> DPDVDECQLMPNACQNGGTCHNSHGGYNCVCVNGWTGEDCSENIDDCASAACFQGATCHDRVASFYCECPHGRTGLLCHLNDACISNPCNEGSNCDTNPVNGKAICTCPSGYTGPACSQDVDECALGANPCEHAGKCLNTLGSFECQCLQGYTGPRCEIDVNECISNPCQND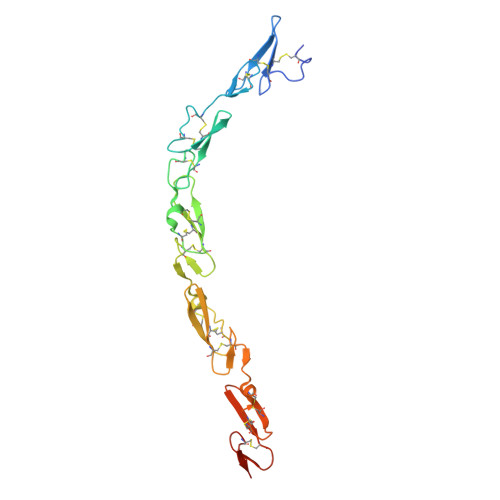ATCLDQIGEFQCICMPGYEGVYCESGRLEVLFQ>MDYLRELYKLEQQAMKLYREASEKARNPEKK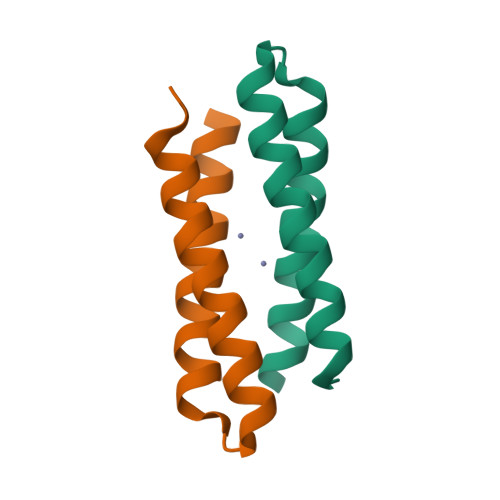SVLQKILEDEEKHIEWLETING[2x]> MTAIVEAPQPGAEAIASPQAAVVAIMAADVQIAVVLDAHAPISVMIDPLLKVVNTRLRELGVAPLEAKGRGRWMLCLVDGTPLRPNLSLTEQEVYDGDRLWLKFLEDTEHRSEVIEHISTAVATNLSKRFAPIDPVVAVQVGATMVAVGVLLGSALLGWWRWQHESWLPAPFAAVIAVLVLTVATMILARSKTVPDRRVGDILLLSGLVPLAVAIAATAPGPVGAPHAVLGFGVFGVAAMLVMRFTGRRLGVYTALVTLCAAATAAGLARMVLLTSAVTLLTCVLLACVLM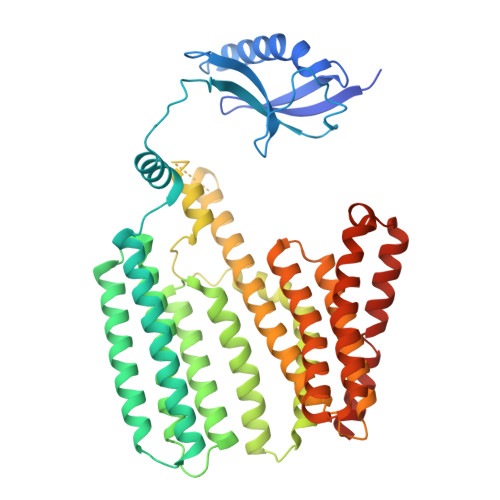YHGAPALSRWLSGIRLPVFPSATSRWVFEARPDLPTTVVVSGGGQPTLEGPASVRDVLLRAERARSFLTGLLVGLGVLTVVCLAGLCDPHAGRRWLPLLLAAFTFGFLILRGRSYVDRWQAITLAATAVLIIAAVAVRYVLVSGSPAVLSAGVAVLVLLPAAGLTAAAVVPNTIYSPLFRKIVEWIEYLCLMPIFPLALWLMNVYEAIRYR>MEQAMRERSELARKGIARAKSVVALAYAGGVLFVAENPSRSLQKISELYDRVGFAAAGKFNEFDNLRRGGIQFADTRGYAYDRRDVTGRQLANVYAQTLGTIFTEQAKPYEVELCVAEVAHYGETKRPELYRITYDGSIADEPHFVVMGGTTEPIANALKESYAENASLTDALRIAVAALRAGSADTSGGDQPTLGVASLEVAVLDANRPRRAFRRITGSALQALLVDQESPQSDGESSG[14x];>XTIVALKYPGGVVMAGDRRSTQGNMISGRDVRKVYITDDYTATGIAGTAAVAVEFARLYAVELEHYEKLEGVPLTFAGKINRLAIMVRGNLAAAMQGLLALPLLAGYDIHASDPQSAGRIVSFDAAGGWNIEEEGYQAVGSGSLFAKSSMKKLYSQVTDGDSGLRVAVEALYDAADDDSATGGPDLVRGIFPTAVIIDADGAVDVPESRIAELARAIIESRSGADTFGSDGGEKHHHHHH[12x];>TTIVALKYPGGVVMAGDRRSTQGNMISGRDVRKVYITDDYTATGIAGTAAVAVEFARLYAVELEHYEKLEGVPLTFAGKIN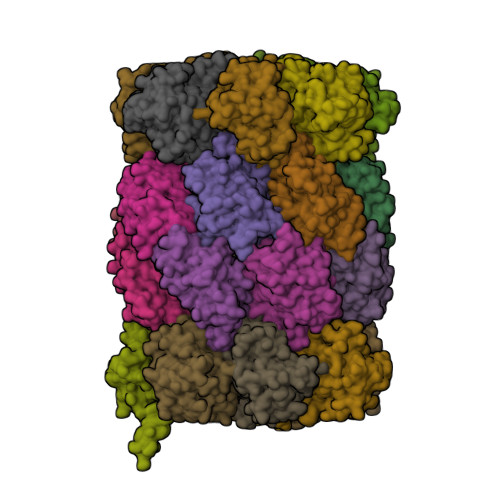RLAIMVRGNLAAAMQGLLALPLLAGYDIHASDPQSAGRIVSFDAAGGWNIEEEGYQAVGSGSLFAKSSMKKLYSQVTDGDSGLRVAVEALYDAADDDSATGGPDLVRGIFPTAVIIDADGAVDVPESRIAELARAIIESRSGADTFGSDGGEKHHHHHH[2x]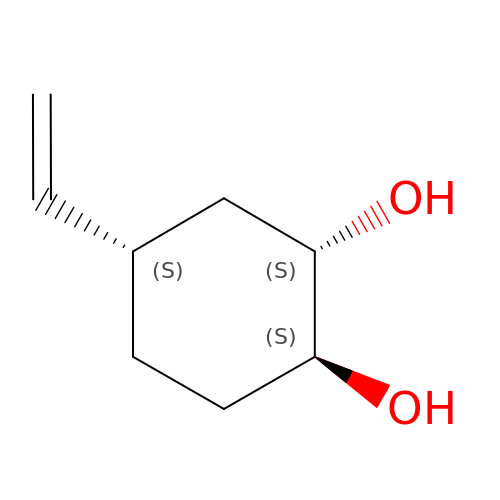(1S,2S,4S)-4-ethenylcyclohexane-1,2-diol | C8 H14 O2 | BSJHRRSHDADBTA-RNJXMRFFSA-N> KLGKLQYSLDYDFQNNQLLVGIIQAAELPALDMGGTSDPYVKVFLLPDKKKKFETKVHRKTLNPVFNEQFTFKVPYSELGGKTLVMAVYDFDRFSKHDIIGEFKVPMNTVDFGHVTEEWRDLQSAEKEEQEKLGDICFSLRYVPTAGKLTVVILEAKNLKKMDVGGLSDPYVKIHLMQNGKRLKKKKTTIKKNTLNPYYNESFSFEVPFE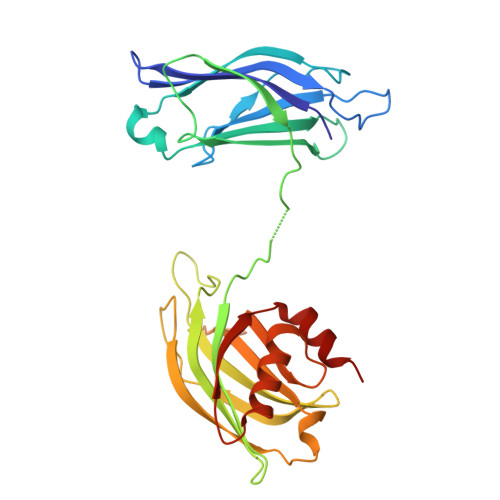QIQKVQVVVTVLDYDKIGKNDAIGKVFVGYNSTGAELRHWSDMLANPRRPIAQWHTLQVEEEVDAMLAVKK>MTSKGPEEEHPSVTLFRQYLRIRTVQPKPDYGAAVAFFEETARQLGLGCQKVEVAPGYVVTVLTWPGTNPTLSSILLNSHTDVVPVFKEHWSHDPFEAFKDSEGYIYARGAQDMKCVSIQYLEAVRRLKVEGHRFPRTIHMTFVPDEEVGGHQGMELFVQRPEFHALRAGFALDEGIANPTDAFTVFYSERSPWWVRV[2x];>NPWWAAFSRVCKDMNL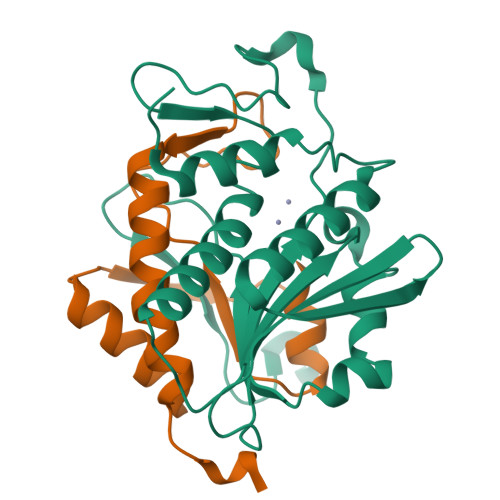TLEPEIMPAAGDNRYIRAVGVPALGFSPMNRTPVLLHDHDERLHEAVFLRGVDIYTRLLPALASVPALPSDS[2x]> MKGCSSYLMYSFGGLLSLWILLVSSTNQCTVRYNVADCSHLKLTHIPDDLPSNITVLNLTHNQLRRLPPTNFTRYSQLAILDAGFNSISKLEPELCQILPLLKVLNLQHNELSQISDQTFVFCTNLTELDLMSNSIHKIKSNPFKNQKNLIKLDLSHNGLSSTKLGTGVQLENLQELLLAKNKILALRSEELEFLGNSSLRKLDLSSNPLKEFSPGCFQTIGKLFALLLNNAQLNPHLTEKLCW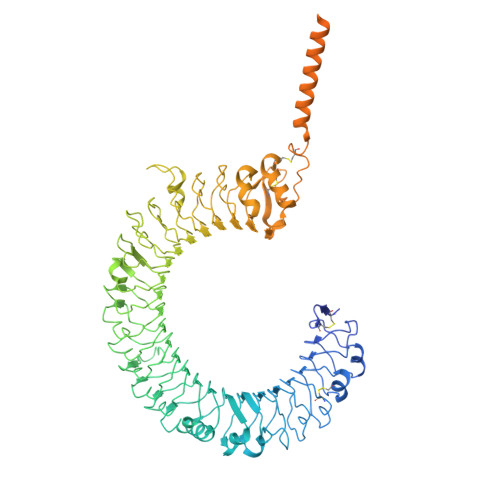ELSNTSIQNLSLANNQLLATSESTFSGLKWTNLTQLDLSYNNLHDVGNGSFSYLPSLRYLSLEYNNIQRLSPRSFYGLSNLRYLSLKRAFTKQSVSLASHPNIDDFSFQWLKYLEYLNMDDNNIPSTKSNTFTGLVSLKYLSLSKTFTSLQTLTNETFVSLAHSPLLTLNLTKNHISKIANGTFSWLGQLRILDLGLNEIEQKLSGQEWRGLRNIFEIYLSYNKYLQLSTSSFALVPSLQRLMLRRVALKNVDISPSPFRPLRNLTILDLSNNNIANINEDLLEGLENLEILDFQHNNLARLWKRANPGGPVNFLKGLSHLHILNLESNGLDEIPVGVFKNLFELKSINLGLNNLNKLEPFIFDDQTSLRSLNLQKNLITSVEKDVFGPPFQNLNSLDMRFNPFDCTCESISWFVNWINQTHTNISELSTHYLCNTPHHYYGFPLKLFDTSSCKDSAPFELLFIISTSMLLVFILVVLLIHIEGWRISFYWNVSVHRILGFKEIDTQAEQFEYTAYIIHAHKDRDWVWEHFSPMEEQDQSLKFCLEERDFEAGVLGLEAIVNSIKRSRKIIFVITHHLLKDPLCRRFKVHHAVQQAIEQNLDSIILIFLQNIPDYKLNHALCLRRGMFKSHCILNWPVQKERINAFHHKLQVALGSRNSAH> MNEMENTVPVLQDDLVSKYERELSTEQEEDTPVILTQLNEDG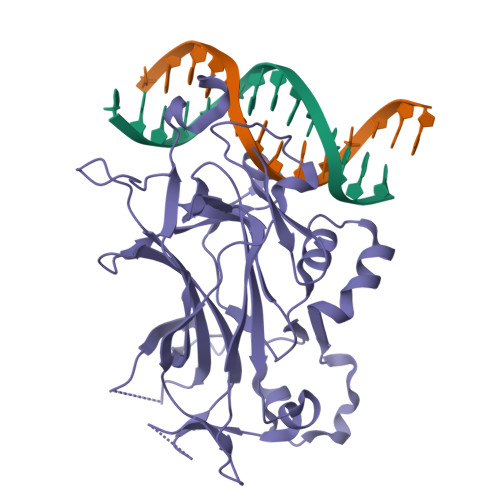TTSNYFDKRKLKIAPRSTLQFKVGPPFELVRDYCPVVESHTGRTLDLRIIPRIDRGFDHIDEEWVGYKRNYFTLVSTFETANCDLDTFLKSSFDLLVEDSSVEGRLRVQYFAIKIKAKNDDDDTEINLVQHTAKRDKGPQFCPSVCPLVPSPLPKHQTIREASNVRNITKMKKYDSTFYLHRDHVNYEEYGVDSLLFSYPEDSIQKVARYERVQFASSISVKKPSQQNKHFSLHVILGAVVDPDTFHGENPGIPYDELALKNGSKGMFVYLQEMKTPPLIIRGRSPSNYASSQRITVR> GPHMKNVDVEFSQAISY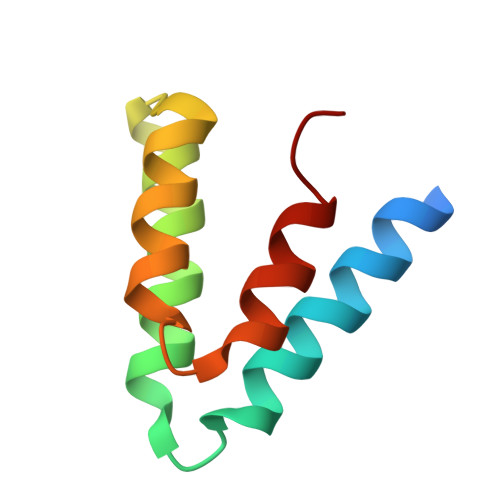VNKIKTRFADQPDIYKHFLEILQTYQREQKPINEVYAQVTHLFQNAPDLLEDFKKFLPD>MTQSLHYSSPRETLTDTIMMAKIRKNLTFEAINQGTGLSLAFVTAALLGQHPLPEQAARVVAEKLDLDEDAIRL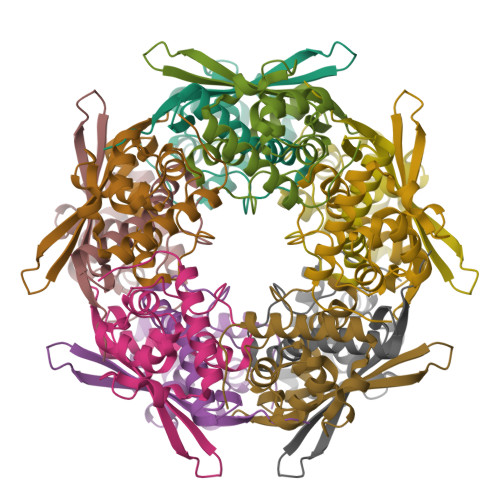LQTIPLRGSIPGGVPTDPTIYRFYEMVQIYGSTLKALVHEQFGDGIISAINFKLDIKKVPDPDGGERAVITLDGKYLPTKPF[5x]In this article, we describe an application of hydrogen deuterium exchange mass spectrometry (HDX‐MS) to identify dynamic regions within type III phosphatidylinositol 4 kinase beta (PI4KIIIβ) in complex with the GTPase Rab11. All deletions were then combined into a single construct that contained two internal deletions, as well as removing the N‐terminus and the C‐terminus. This construct, referred to from now on as xtalPI4K (HsPI4KB S294A 121–784, Δ249–287, Δ408–507), enabled us to generate crystals of PI4KIIIβ in complex with Rab11.

The higher resolution crystals of the PI4KIIIβ bound to GTPγS‐Rab11 revealed novel molecular details of the PI4KIIIβ‐Rab11 interface. These crystals revealed formation of a helical element (residues 70–77) within switch 2 (residues 72–82) of Rab11 that was not present in structures of Rab11 GTPγS alone. To examine if this conformational change occurs in solution, we examined the H/D exchange information of Rab11 in the presence and absence of PI4KIIIβ, mapped on to the structure. Notably, there was a decrease in exchange in the region from 72 to 80 within switch 2 of Rab11 [Fig. 6(A)], and there is no direct contact between this region and PI4KIIIβ. Intriguingly, the combined crystallographic and dynamic information from HDX‐MS revealed conformational changes in the switch region of Rab11 upon PI4KIIIβ binding. Switch plasticity in Rab11 binding interactions has been noted for a number of Rab11 effector complexes, specifically in Rab11 bound to the motor protein myosin V,30 as well as in the complex of Rab11 with FIP3.42 This intriguing observation that PI4KIIIβ changes the conformation of the Rab11 switch regions both in solution and in the crystal structure, suggests that this may be a mechanism of how Rab11 could be biased toward binding specific effectors. The fully optimized xtalPI4KIIIβ construct in complex with Rab11 formed crystals in the absence of small molecule inhibitors, and crystallization was amenable to soaking with a variety of small molecule inhibitors.

> GSHMQNNSAKQSWLLRLFESKLFDISMAISYLYNSKEPGVQAYIGNRLFCFRNEDVDFYLPQLLNMYIHMDEDVGDAIKPYIVHRCRQSINFSLQCALLLGAYSSDMHISTQRHSRGTKLRKLILSDELKPANLKRTAANPKVENEDEPVRLAPEREFIKSLMAIGKRLATLPTKEQKTQRLISELSLLNHKLPARVWLPTAGFDHHVVRVPHTQAVVLNSKDKAPYLIYVEVLECENFDTTSVPARIPENRRDPEDPSAVALKEPWQEKVRRIREGSPYGHLPNWRLLSVIVKCGDDLRQELLAFQVLKQLQSIWEQERVPLWIKPYKILVISADSGMIEPVVNAVSIHQVKKQSQLSLLDYFLQEHGSYTTEAFLSAQRNFVQSCAGYCLVCYLLQVKDRHNGNILLDAEGHIIHIDFGFILSSSPRNLGFETSAFKLTTEFVDVMGGLDGDMFNYYKMLMLQGLIAARKHMDKVVQIVEIMQQGSQLPCFHGSSTIRNLKERFHMSMTEEQLQLLVEQMVDGSMRS;> GSHMGTRDDEYDYLFKVVLIGDSGVGKSNLLSRFTRNEFNLESKSTIGVEFATRSIQVDGKTIKAQIWDTAGLERYRAITSAYYRGAVGALLVYDIAKHLTYENVERWLKELRDHADSNIVIMLVGNKSDLRHLRAVPTDEARAFAEKNGLSFIETSALDSTNVEAAFQTILTEIYRIVSQKQMSDRRENDMSPSNNVVPIHVPPTTENKPKVQCCQNI S-[2-[3-[[(2R)-4-[[[(2R,3S,4R,5R)-5-(6-aminopurin-9-yl)-4-oxidanyl-3-phosphonooxy-oxolan-2-yl]methoxy-oxidanyl-phosphoryl]oxy-oxidanyl-phosphoryl]oxy-3,3-dimethyl-2-oxidanyl-butanoyl]amino]propanoylamino]ethyl] (5Z,8Z,11Z,14Z)-icosa-5,8,11,14-tetraenethioate | C41 H66 N7 O17 P3 S | 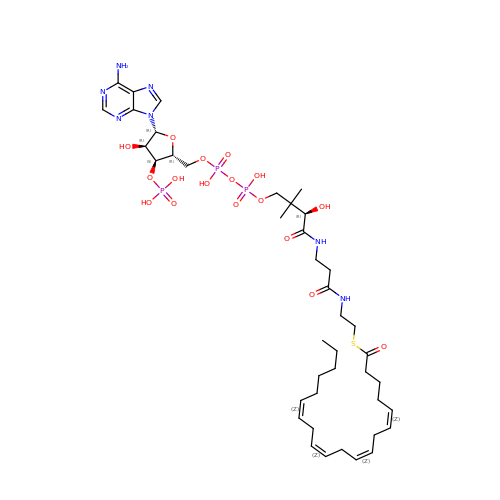JDEPVTUUCBFJIW-YQVDHACTSA-N>MFEARLVQGSILKKVLEALKDLINEACWDISSSGVNLQSMDSSHVSLVQLTLRSEGFDTYRCDRNLAMGVNLTSMSKILKCAGNEDIITLRAEDNADTLALVFEAPNQEKVSDYEMKLMDLDVEQLGIPEQEYSCVVKMPSGEFARICRDLSHIGDAVVISCAKDGVKFSASGELGNGNIKLSQTSNVDKEEEAVTIEMNEPVQLTFALRYLNFFTKATPLSSTVTLSMSADVPLVVEYKIADMGHLKYYLAPKIEDEEGS[3x];>GIQGLAKLIADVAPSAIRENDIKSYFGRKVAIDASMSIYQFLIAVRQGGDVLQNEEGETTSHLMGMFYRTIRMMENGIKPVYVFDGKPPQLKSGELAKRSERRAEAEKQLQQAQAAGAEQEVEKFTKRLVKVTKQHNDECKHLLSLMGIPYLDAPSEAEASCAALVKAGKVYAAATEDMDCLTFGSPVLMRHLTASEAKKLPIQEFHLSRILQELGLNQEQFVDLCILLGSDYCESIRGIGPKRAVDLIQKHKSIEEIVRRLDPNKYPVPENWLHKEAHQLFLEPEVLDPESVELK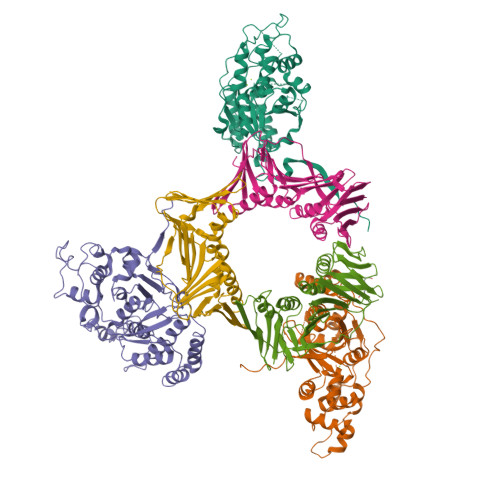WSEPNEEELIKFMCGEKQFSEERIRSGVKRLSKSRQGSTQGRLDDFFKVTGSLSSAKRKEPEPKGSTKKKAKTGAAGKFKRGK[3x]>SMAKIIFPEDFIWGAATSSYQIEGAFNEDGKGESIWDRFSHTPGKIENGDTGDIACDHYHLYREDIELMKEIGIRSYRFSTSWPRILPEGKGRVNQKGLDFYKRLVDNLLKANIRPMITLYHWDLPQALQDKGGWTNRDTAKYFAEYARLMFEEFNGLVDLWVTHNEPWVVAFEGHAFGNHAPGTKDFKTALQVAHHLLLSHGMAVDIFREEDLPGEIGITLNLTPAYPAGDSEKDVKAASLLDDYINAWFLSPVFKGSYPEELHHIYEQNLGAFTTQPGDMDIISRDIDFLGINYYS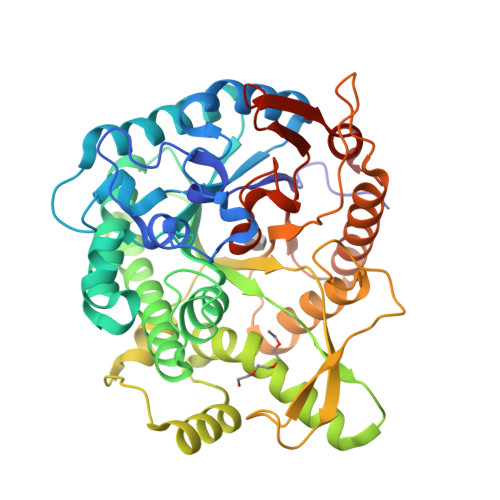RMVVRHKPGDNLFNAEVVKMEDRPSTEMGWEIYPQGLYDILVRVNKEYTDKPLYITENGAAFDDKLTEEGKIHDEKRINYLGDHFKQAYKALKDGVPLRGYYVWSLMDNFEWAYGYSKRFGLIYVDYENGNRRFLKDSALWYREVIEKGQVEAN[2x]> MRQSQLYPNLGYNNQNGQFNYLPSPEQQSIYRNNIQTPTSGISNNLFPLQSQQRIIQPQYHYQTPLINNNIINNNNNINNNNIVYQQDQQTQPQAQPQQQPQQTQTQSPSQQEKEQEQQQQELKEQQQKQQQQQEQEQQELMRQKKTNSLLSITPFNKEEDLKKIFLNSIESIDSSIDKVATIPDPTLKVLYKRDPGFNYFDGGSYFWSTLVIEKHIELPQEITNGYLSTSTKSLLGLFPEIGRAWISIDQTLYLWDYRDSGELISHNLSQIITNCALIQPKKNTFKDAVKKVMVVCTHVEIFLFALCYSNETKFEILSTLSIPSDNIFITDIVGTKEGRIFLSGQDGNIYEIEYSKDNLFWFSNEKIKKINLTQTFFNSFINLSKKKEIIQLIYDEDRYLLYSLSKDSTINVYSLGKIGDKFEHLKTIYPINDIDSLFNNNINNNNNNNNYYSQQYQYQQQQQNQQYQQSQYGQQQQQQQPNQYGQQQQQQQPLQQQQQQQQQQQQNFSRKNMVIMSIHISPKETEFNFIAILSSGERLYYTLNRLAYIRSPPNNVDNNGNSNIHYTYYSNGVFFTASEVSDQEDRLVGTTLFGNDIIKSHYETSKSGFSNQISQDTLSEKSNLFSIRGRVSVIKEDIVNDGKPTVYYKELSNEHMNTPRRFLCLNSLGLHFISKLRYVDLLQNILSSNNPQDIDNFFDAFGKIIASSLCISLYCSSPHSSILLHDQVYSGISIPKTTTTRIADLAMTFLRRKSGKPQYYQPVVIQQMFGDMGAPVNKTELMYSNAYNGLLAYLARVLYPLWNQSVVTSAGCSYWSIVQLQLFQSHLSNLLSFLDISQLIPKGQEIPIIKIATNKTSSTTTTTTTANNSSSNEIYGEDEAIKNEKRSLIGLKNIIVKSIQILNLFLILSQYNFKQLFDSSSIELDIKRKIDLLKFRDILNSDILGKNLPLPTISSLTTSTTTTTTTTTTSTTSSSSSSTSPLTTSTSNSTLTLLIDSLMKTLNSHNINIDQVSNQLETECPIFFKKENRELYKVKEKLNMVLRDGSTYFTDSLVKDSALILDSISPNYNLSEIVDLFIAIKAFNYVTP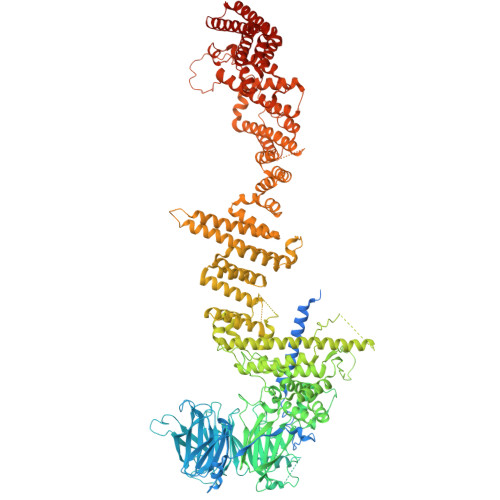LCLQYAQDLDPRGITLIPSNNPSDEFKLKLSQKKSTFQEIIKLLNFIQSDNNNNNNNSGGGGGDNNNYNNTFEIIDIIIQQVLVCQDRLAHEMIYSWILNNGMTSKFFEINTPFITEFLFANDIDLCWKVLAKHQELLKAVHVLFQIAERSTTLDEKILAYTNCTMILSEQKDEDAYIQAKNQITFANIQKQIVLQLENYLNNPNESNNRNNSSNNNGGQPFDINQIKESISNLNKTIFDITTLFTDYARKYYLHEQMLYLCHIGNHSDQNFIQILWKIIIDKEIPPPSSNLSLDDNAENDDGLKISVGGVIESLVSKISNIGYDFYPNEITFPVEFIINYGERAIFNFSRNKSEAEKKEISPNWLTSSLHDHVKIDYWILVDYYNNTIEKGSWKEEDESLIYITSVYFYLVESLINTIQTATERRLFSSKQILQSLENRESTFKSIFNRQRSSLNQETIKKLEQLLIKFEKIISISKSFKDFRGY>[2x]HHHHHHFNLPPGNYKKPKLLYCSNGGHFLRILPDGTVDGTRDRSDQHIQLQLSAESVGEVYIKSTETGQYLAMDTDGLLYGSQTPNEECLFLERLEENHYNTYISKKHAEKNWFVGLKK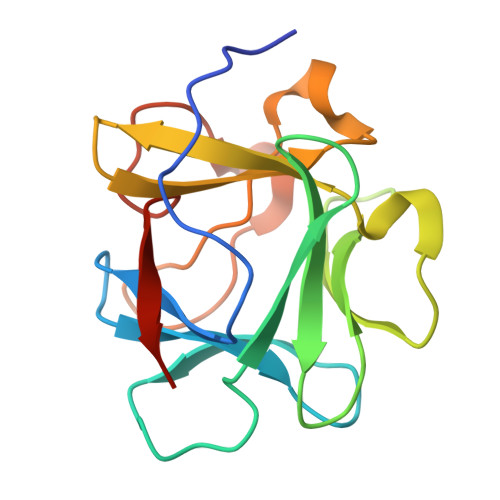NGSVKRGPRTHYGQKAILFLPLPVSSD> APYVYANAKALQDTEKVGNHHQCVELIQHYIRVGQASTWQQGAAVFGNKNIEVGTVIATFVNGRYPNHNSGNHAAFFLGQDTGGIWVMDQWKDDIAKPRVSKRYIRKLHNGSVRSDGTYIRMSNNAEAYFIVE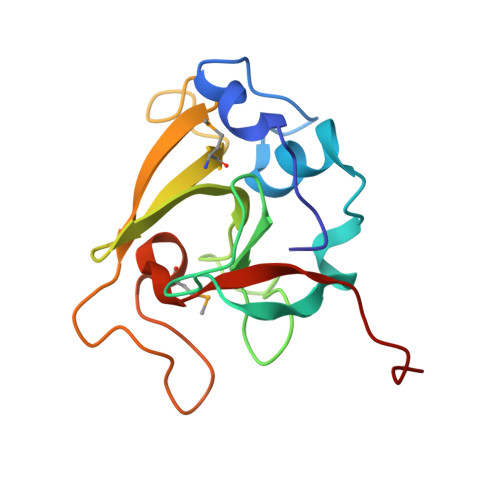LEHHHHH>[4x]MANLHALRREQRAQGPATIMAIGTATPPNLYEQSTFPDFYFRVTNSDDKQELKKKFRRMCEKTMVKKRYLHLTEEILKERPKLCSYKEASFDDRQDIVVEEIPRLAKEAAEKAIKEWGRPKSEITHLVFCSISGIDMPGADYRLATLLGLPLTVNRLMIYSQACHMGAAMLRIAKDLAENNRGARVLVVACEITVLSFRGPNEGDFEALAGQAGFGDGAGAVVVGADPLEGIEKPIY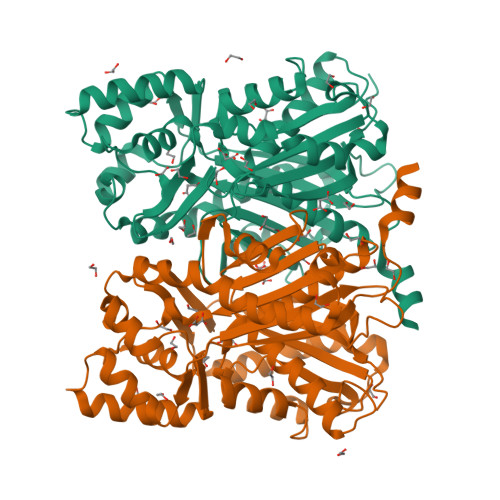EIAAAMQETVAESQGAVGGHLRAFGWTFYFLNQLPAIIADNLGRSLERALAPLGVREWNDVFWVAHPGNWAIIDAIEAKLQLSPDKLSTARHVFTEYGNMQSATVYFVMDELRKRSAVEGRSTTGDGLQWGVLLGFGPGLSIETVVLRSMPLHHHH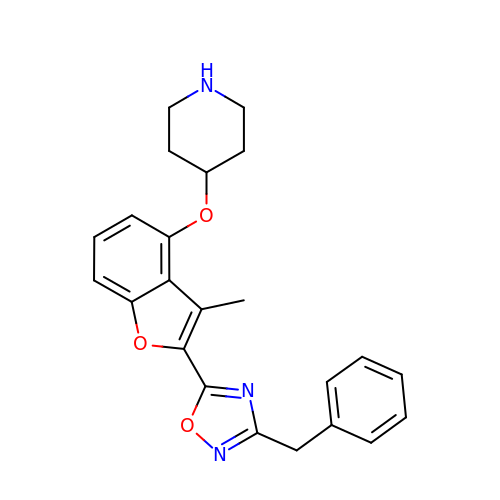4-{[2-(3-benzyl-1,2,4-oxadiazol-5-yl)-3-methyl-1-benzofuran-4-yl]oxy}piperidine | C23 H23 N3 O3 | QVBWWXFSCCHYFK-UHFFFAOYSA-N>MPSETPQAEVGPTGCPHRSGPHSAKGSLEKGSPEDKEAKEPLWIRPDAPSRCTWQLGRPASESPHHHTAPAKSPKILPDILKKIGDTPMVRINKIGKKFGLKCELLAKCEFFNAGGSVKDRISLRMIEDAERDGTLKPGDTIIEPTSGNTGIGLALAAAVRGYRCIIVMPEKMSSEKVDVLRALGAEIVRTPTNARFDSPESHVGVAWRLKNEIPNSHILDQYRNASNPLAHYDTTADEILQQCDGKLDMLVASVGTGGTITGIARKLKEKCPGCRIIGVDPEGSILAEPEELNQTEQTTYEVEGIGYDFIPTVLDRTVVDKWFKSNDEEAFTFARMLIAQEGLLCGGSAGSTVAVAVKAAQELQEGQRCVVILPDSVRNYMTKFLSDRWMLQKGFLKEEDLTEKKPWWWHLRVQELGLSAPLTVLPTITCGHTIEILREKGFDQAPVVDEAGVILGMVTLGNMLSSLLAGKVQPSDQVGKVIYKQFKQIRLTDTLGRLSHILEMDHFALVVHEQIQYHSTGKSSQRQMVFGVVTAIDLLNFVAAQERDQKAAHHHHHH[8x]

Cystathionine beta-synthase (CBS) is an essential metabolic enzyme across all domains of life for the production of glutathione, cysteine, and hydrogen sulfide. Human CBS adopts a unique multi-domain structure: an N-terminal haem binding domain (residues 38–74), a central PLP-dependent catalytic domain (CD, residues 75–382), and a C-terminal regulatory domain (RD, residues 411–551)5,11,12. The RD adopts the evolutionarily conserved Bateman module, consisting of two tandem CBS motifs (CBS-1 and CBS-2) and a surface-exposed loop (residues 516–525) extending from a CBS-2 motif. Here we show using cryo-electron microscopy that full-length human CBS in the basal and SAM-bound activated states polymerises as filaments mediated by a conserved regulatory domain loop.

We pursued the cryo-EM structure of full-length CBS initially using two constructs: one where an N-terminal His-tag was removed during purification (CBSFL) and one with a permanent C-terminal His-tag (CBSFL-CHis). Micrographs of full-length CBS from both constructs in vitreous ice clearly showed the presence of flexible filaments of varying lengths agreeing with 2D classes. Multiple maps were processed using both helical and single particle reconstruction to resolutions of between 3.9 and 3.0 Å. Both constructs resulted in maps with virtually identical conformations, and both were used for modelling. The CBS filament adopts a left-handed helical architecture with a twist of −108° and a rise of 51 Å. In the basal state, CBS regulatory domains sterically block the catalytic domain active site, resulting in a low-activity filament with three CBS dimers per turn. The domain-swapped dimer, previously observed in crystal structures, is the repeating unit, and helical formation is driven by inter-dimeric RD interactions, i.e., between the RDs of neighbouring subunits of the filament. Loop 516–525, a β-turn-β extension from the CBS-2 motif in the conserved Bateman module, plays a key role in driving oligomerisation. Specifically, one RD each from two neighbouring CBS dimers interact in a butterfly-like dimeric arrangement, related by C2 symmetry, such that the loop 516–525 from an RD of one dimer forms a clasp around an RD of the neighbouring dimer. We also found that CBSFL-CHis is more thermostable than CBSFL by ~3 °C, possibly because it is forming longer oligomers and is less degraded than CBSFL. Though we do not know the exact reason for this phenomenon, this difference is likely due to the longer oligomers and stabilising effect of the C-terminal His-tag.>[4x]MSQPITRENFDEWMIPVYAPAPFIPVRGEGSRLWDQQGKEYIDFAGGIAVNALGHAHPELREALNEQASKFWHTGNGYTNEPVLRLAKKLIDATFADRVFFCNSGAEANEAALK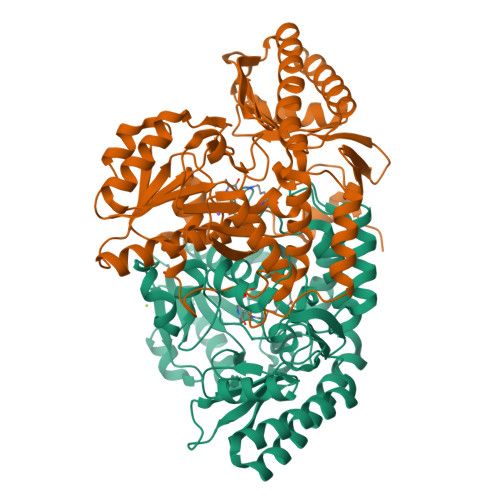LARKFAHDRYGSHKSGIVAFKNAFHGRTLFTVSAGGQPAYSQDFAPLPADIRHAAYNDINSASALIDDSTCAVIVEPIQGEGGVVPASNAFLQGLRELCNRHNALLIFDEVQTGVGRTGELYAYMHYGVTPDLLTTAKALGGGFPVGALLATEECARVMTVGTHGTTYGGNPLASAVAGKVLELINTPEMLNGVKQRHDWFVERLNTINHRYGLFSEVRGLGLLIGCVLNADYAGQAKQISQEAAKAGVMVLIAGGNVVRFAPALNVSEEEVTTGLDRFAAACEHFVSRGSS> MKFYIDDLPVLFPYPKIYPEQYNYMCDIKKTLDVGGNSILEMPSGTGKTVSLLSLTIAYQMHYPEHRKIIYCSRTMSEIEKALVELENLMDYRTKELGYQEDFRGLGLTSRKNLCLHPEVSKERKGTVVDEKCRRMTNGQAKRKLEEDPEANVELCEYHENLYNIEVEDYLPKGVFSFEKLLKYCEEKTLCPYFIVRRMISLCNIIIYSYHYLLDPKIAERVSNEVSKDSIVIFDEAHNIDNVCIESLSLDLTTDALRRATRGANALDERISEVRKVDSQKLQDEYEKLVQGLHSADILTDQEEPFVETPVLPQDLLTEAIPGNIRRAEHFVSFLKRLIEYLKTRMKVLHVISETPKSFLQHLKQLTFIERKPLRFCSERLSLLVRTLEVTEVEDFTALKDIATFATLISTYEEGFLLIIEPYEIENAAVPNPIMRFTCLDASIAIKPVFERFSSVIITSGTISPLDMYPRMLNFKTVLQKSYAMTLAKKSFLPMIITKGSDQVAISSRFEIRNDPSIVRNYGSMLVEFAKITPDGMVVFFPSYLYMESIVSMWQTMGILDEVWKHKLILVETPDAQETSLALETYRKACSNGRGAILLSVARGKVSEGIDFDHQYGRTVLMIGIPFQYTESRILKARLEFMRENYRIRENDFLSFDAMRHAAQCLGRVLRGKDDYGVMVLADRRFSRKRSQLPKWIAQGLSDADLNLSTDMAISNTKQFLRTMAQPTDPKDQEGVSVWSYEDLIKHQNSRKDQGGFIENENKEGEQDEDEDEDIEMQ;> MSHSGAAIFEKVSGIIAINEDVSPAELTWRSTDGDKVHTVVLSTIDKLQATPASSEKMMLRLIGKVDESKKRKDNEGNEVVPKPQRHMFSFNNRTVMDNIKMTLQQIISRYKDADIYEEKRRREESAQHTETPMSSSSVTAGTPTPHLDTPQLNNGAPLINTAKLDDSLSKEKLLTNLKLQQSLLKGNKVLMKVFQETVINAGLPPSEFWSTRIPLLRAFALSTSQKVGPYNVLSTIKPVASSENKVNVNLSREKILNIFENYPIVKKAYTDNVPKNFKEPEFWARFFSSKLFRKLRGEKIMQNDRGDVIIDRYLTLDQEFDRKDDDMLLHPVKKIIDLDGNIQDDPVVRGNRPDFTMQPGVDINGNSDGTVDILKGMNRLSEKMIMALKNEYSRTNLQNKSNITNDEEDEDNDERNELKIDDLNESYKTNYAIIHLKRNAHEKTTDNDAKSSADSIKNADLKVSNQQMLQQLSLVMDNLINKLDLNQVVPNNEVSNKINKRVITAIKINAKQAKHNNVNSALGSFVDNTSQANELEVKSTLPIDLLESCRMLHTTCCEFLKHFYIHFQSGEQKQASTVKKLYNHLKDCIEKLNELFQDVLNGDGESMSNTCTAYLKPVLNSITLATHKYDEYFNEYNNNSN;> MSDYSLKHSVTQYLEEIPQQVQNRLYTSPATCLAIYRILPPLAKFFIMAMVFNENEVPLLDLDKWVNSNGKLQFQNAIKSMKSLHLLIPNKSSGTLMINLNPTFKISLRNALTGGEVQNSFGVVVEENVVSLDLLDEYSANKWETILHFMVGTPLAKIPSEKVLNLLKHSKLMEEVNSTGEFKITNEGFQFLLQEINSQLWTLLLQYLKMIETSKMDLVDVLHFIFMLGALEVGKAYKIDALSETQRIMLQDMRDYGLVFQKHSNDSIFYPTKLALMLTSDTKTIRSASNAMDSVLRQNREEPSVNEDGANGKSTTDITTSDDLNKAGLKNQDIPDGSLIVETNFKIYSYSNSPLQIAVLSLFVHLKARFVNMVLGQITRESIRRALTNGITADQIIAYLETHAHPQMRRLAEEKLEKKLELDPNCKEPLQVLPPTVVDQIRLWQLELDRVITYEGSLYSDFETSQEYNLLSKYAQDIGVLLWKDDKKKKFFISKEGNSQVLDFAKRKLKKKQ;> MDAISDPTFKHARSRKQVTEESPSLLTVIIEIAPKLWTTFDEEGNEKGSIIKVLEALIVFLNAHLAFNSANKVAVIAAYSQGIKYLYPESTSALKASESENKTRSDLKIINSDMYRRFRNVDETLVEEIYKLFELEKKQIEQNSQRSTLAGAMSAGLTYVNRISKESVTTSLKSRLLVLTCGSGSSKDEIFQYIPIMNCIFSATKMKCPIDVVKIGGSKESTFLQQTTDATNGVYLHVESTEGLIQYLATAMFIDPSLRPIIVKPNHGSVDFRTSCYLTGRVVAVGFICSVCLCVLSIIPPGNKCPACDSQFDEHVIAKLKRKPVVPRLKAKKKVTKP;> ARARKGALVQCDPSIKALILQIDAKMSDIVLEELDDTHLLVNPSKVEFVKHELNRLLSKNIYNPMD;> MAPVVISESEEDEDRVAITRRTKRQVHFDGEGDDRVDQQQQQHSSSHRDRDKHVQRKKKKRLSNRNLQGSNGGYAWEDEIKRSWDLVKVDDEGDMASLVASIVEARKKRTAKKNITPYQRGIIRSLILTLDCSEAMLEKDLRPNRHAMIIQYAIDFVHEFFDQNPISQMGIIIMRNGLAQLVSQVSGNPQDHIDALKSIRKQEPKGNPSLQNALEMARGLLLPVPAHCTREVLIVFGSLSTTDPGDIHQTIDSLVSEKIRVKVLGLSAQVAICKELCKATNYGDESFYKILLDETHLKELFNEAVTPLPVNKINKGFTLVKMGFPTRIFEDTPTFCSCHSKLVYGGYFCPNCHSKVCSLPTVCPCCDLMLILSTHLARSYHHLMPLKTFAEVPTTEKFRSEDCFSCQSRFPILKNHKNGKLLTSSRYRCEDCKQEFCVDCDVFIHEILHNCPGCESKPVIT;> MTDVEGYQPKSKGKIFPDMGESFFSSDEDSPATDAEIDENYDDNRETSEGRGERDTGAMVTGLKKPRKKTKSSRHTAADSSMNQMDAKDKALLQDTNSDIPADFVPDSVSGMFRSHDFSYLRLRPDHASRPLWISPSDGRIILESFSPLAEQAQDFLVTIAEPISRPSHIHEYKITAYSLYAAVSVGLETDDIISVLDRLSKVPVAESIINFIKGATISYGKVKLVIKHNRYFVETTQADILQMLLNDSVIGPLRIDSDHQVQPPEDVLQQQLQQTAGKPATNVNPNDVEAVFSAVIGGDNEREEEDDDIDAVHSFEIANESVEVVKKRCQEIDYPVLEEYDFRNDHRNPDLDIDLKPSTQIRPYQEKSLSKMFGNGRARSGIIVLPCGAGKTLVGITAACTIKKSVIVLCTSSVSVMQWRQQFLQWCTLQPENCAVFTSDNKEMFQTESGLVVSTYSMVANTRNRSHDSQKVMDFLTGREWGFIILDEVHVVPAAMFRRVVSTIAAHAKLGLTATLVREDDKIGDLNFLIGPKLYEANWMELSQKGHIANVQCAEVWCPMTAEFYQEYLRETARKRMLLYIMNPTKFQACQFLIQYHERRGDKIIVFSDNVYALQEYALKMGKPFIYGSTPQQERMNILQNFQYNDQINTIFLSKVGDTSIDLPEATCLIQISSHYGSRRQEAQRLGRILRAKRRNDEGFNAFFYSLVSKDTQEMYYSTKRQAFLVDQGYAFKVITHLHGMENIPNLAYASPRERRELLQEVLLKNEEAAGIEVGDDADNSVGRGSNGHKRFKSKAVRGEGSLSGLAGGEDMAYMEYSTNKNKELKEHHPLIRKMYYKNLKK;> MNEDLPKEYFELIRKALNEKEAEKAPLSRRRRVRRKNQPLPDAKKKFKTGLNELPRESVVTVNLDSSDDGVVTVPTDDSVEEIQSSEEDYDSEEFEDVTDGNEVAGVEDISVEIKPSSKRNSDARRTSRNVCSNEERKRRKYFHMLYLVCLMVHGFIRNEWINSKRLSRKLSNLVPEKVFELLHPQKDEELPLRSTRKLLDGLKKCMELWQKHWKITKKYDNVGLYMRTWKEIEMSANNKRKFKTLKRSDFLRAVSKGHGDPDISVQGFVAMLRACNVNARLIMSCQPPDFTNMKIDTSLNGNNAYKDMVKYPIFWCEVWDKFSKKWITVDPVNLKTIEQVRLHSKLAPKGVACCERNMLRYVIAYDRKYGCRDVTRRYAQWMNSKVRKRRITKDDFGEKWFRKVITALHHRKRTKIDDYEDQYFFQRDESEGIPDSVQDLKNHPYYVLEQDIKQTQIVKPGCKECGYLKVHGKVGKVLKVYAKRDIADLKSARQWYMNGRILKTGSRCKKVIKRTVGRPKGEAEEEDERLYSFEDTELYIPPLASASGEITKNTFGNIEVFAPTMIPGNCCLVENPVAIKAARFLGVEFAPAVTSFKFERGSTVKPVLSGIVVAKWLREAIETAIDGIEFIQEDDNRKEHLLGALESWNTLLLKLRIRSKLNSTYGKIAEEEPNVTKEQNIADNHDNTETFMGGGFLPGIANHEARPYSEPSEPEDSLDYVSVDKAEESATDDDVGEDYSDFMKELEMSEESD;> MSKSTNVSYERVELFENPKVPIEVEDEILEKYAESSLDHDMTVNELPRFFKDLQLEPTIWKLVRNEDVIIEGTDVIDFTKLVRCTCQLLILMNNLTVIDDLWSMLIRNCGRDVDFPQVALRDHVLSVKDLQKISNLIGADQSSGTIEMISCATDGKRLFMTYLDFGCVLGKLGYLKM

The versatile nucleotide excision repair (NER) pathway initiates as the XPC–RAD23B–CETN2 complex first recognizes DNA lesions from the genomic DNA and recruits the general transcription factor complex, TFIIH, for subsequent lesion verification. Here, we present a cryo-EM structure of an NER initiation complex containing Rad4–Rad23-Rad33 (yeast homologue of XPC–RAD23B–CETN2) and 7-subunit coreTFIIH assembled on a carcinogen-DNA adduct lesion at 3.9–9.2 Å resolution. The coreTFIIH contains two helicase-family ATPase subunits: XPB(Ssl2) and XPD(Rad3) in human(yeast), and 5 nonenzymatic subunits: p62(Tfb1), p52(Tfb2), p44(Ssl1), p34(Tfb4), and p8(Tfb5). Altogether, our study illustrates how the Rad4–Rad23–Rad33 (XPC–RAD23B–CETN2) complex recruits TFIIH to damaged DNA in 3D structural models and provides the groundwork to visualize how the NER initiation is carried out in multiple, coordinated yet distinct steps.

To better resolve the disordered density, we refined a less populated class containing Rad4–Rad33/DNA at 9.2 Å resolution (Map 2, EMDB-22588), as well as a class containing Rad4 BHD3 (but not including BHD1-2 and TGD)-Rad33-DNA at 7.9 Å resolution (Map 3, EMDB-22576). Although the main body of Rad4 (residues 123–632) was in close proximity to the C-terminal helicase domain of Ssl2 (C-Ssl2, residues 549–776), it apparently had little direct contact with C-Ssl2. However, an unassigned EM density bridging C-terminal end of Rad4 BHD3 (residue 632) and C-Ssl2 indicated the presence of Rad33: Rad33 and human centrin 2 (CETN2) are both EF-hand calcium-binding proteins that interact with the conserved C-terminal region of Rad4 and XPC, respectively, and stimulate NER activity. To resolve this region, we further refined this map up to ~7.9 Å resolution (Map 3) using a mask that excludes the TGD and BHD1 domains of Rad4. This allowed us to reliably dock a homology model of the Rad33 C-terminal lobe (residues 94–169) bound to the Rad4 C-terminal region (C-Rad4; residues 648–664) into the corresponding density, guided by cross-links of high confidence between C-Rad4 and the C-terminal region of Ssl2 (e.g., Rad4 S660–Ssl2 K796). The N-terminal lobe of Rad33 (residues 26–93) was not observed in the map. The conserved hydrophobic surface of C-Rad4 consisting of Thr651, Ile658, Leu66271 pack against hydrophobic residues of BHD3 (Phe585, Leu586, Thr624). Our model suggests that this is due to the role of C-XPC (Rad4) in binding to CETN2 (Rad33) which in turn directly interacts with the C-terminal helix of XPB (Ssl2). By contrast, the same superposition showed that Rad33 and XPA(Rad14) would encounter steric clash with each other as both bind to the C-terminal helix of C-Ssl2. This suggests that Rad33 and Rad14 are mutually exclusive when they bind to Ssl2.>GPGSMSGIDPKRFGKVAVLLGGDSAEREVSLNSG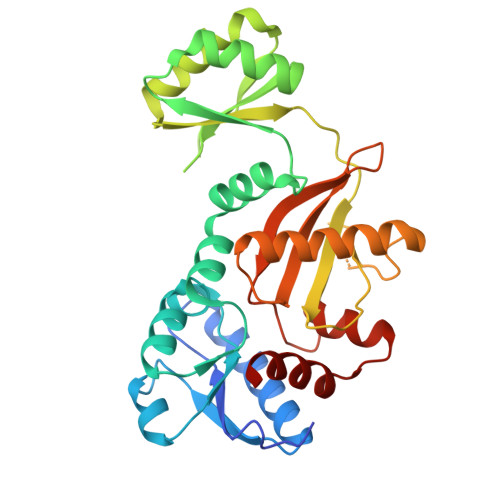RLVLQGLRDAGIDAHPFDPAQRPLAALKDEGFVRAFNALHGGYGENGQIQGALDFYGIRYTGSGVLGSALGLDKFRTKLVWQQTGIPTPPFETVMRGDDYAARAQDIVAKLGVPLFVKPASEGSSVAVEKVKSADALPAALEEAAKHDKIVIVEKSIEGGGEYTACIAADLDLPLIRIVPAGEFYDYHAKYIANDTQYLIPCGLDAAKEAEFKRIARRAFDVLGCTDWGRADFMLDAAGNPYFLEVNTAPGMTDHSLPPKAARAVGIGYSELVVKVLSLTLD[4x]> MKEFYISIETVGNNIVERYIDENGKERTREVEYLPTMFRHCKEESKYKDIYGKNCAPQKFPSMKDARDWMKRMERIGLEALGMNDFKLAYISDTYGSEIVYDRKFVRVANCDIEVTGDKFPDPMKAEYEIDAITHYDSIDDRFYVFDLLNSMYGSVSKWDAKLAAKLDCEGGDEVPQEILDRVIYMPFDNERDMLMEYINLWEQKRPAIFTGWNIEGFAVPYIMNRVKMILGERSMKRFSPIGRVKSKLIQNMYGSKEIYSIDGVSILDYLDLYKKFAFTNLPSFSLESVAQHETKKGKLPYDGPINKLRETNHQRYISYNIIDVESVQAIDKIRGFIDLVLSMS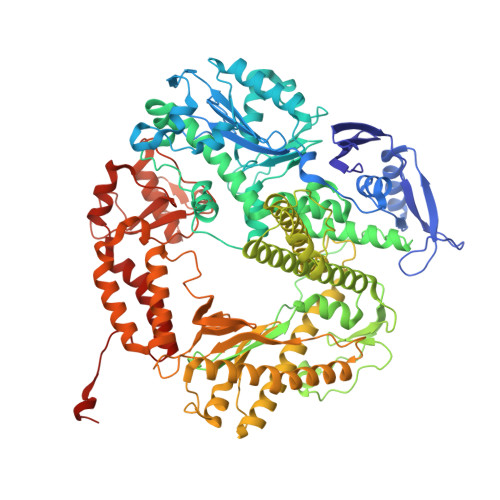YYAKMPFSGVMSPIKTWDAIIFNSLKGEHKVIPQQGSHVKQSFPGAFVFEPKPIARRYIMSFDLTSLYPSIIRQVNISPETIRGEFEVHPIHEYIAGTAPKPSDEYSCSPNGWMYDKHQEGIIPKEIAKVFFQRKDWKKKMFAEEMNAEAIKKIIMKGAGSCSTKPEVERYVKFSDDFLNELSNYTESVLNSLIEECEKAATLANTNQLNRKILINSLYGALGNIHFRYYDLRNATAITIFGQVGIQWIARKINEYLNKVCGTNDEDFIAAGDTDSVYVCVDKVIEKVGLDRFKEQNDLVEFMNQFGKKKMEPMIDVAYRELCDYMNNREHLMHMDREAISCPPLGSKGVGGFWKAKKRYALNVYDMEDKRFAEPHLKIMGMETQQSSTPKAVQEALEESIRRILQEGEESVQEYYKNFEKEYRQLDYKVIAEVKTANDIAKYDDKGWPGFKCPFHIRGVLTYRRAVSGLGVAPILDGNKVMVLPLREGNPFGDKCIAWPSGTELPKEIRSDVLSWIDHSTLFQKSFVKPLAGMCESAGMDYEEKASLDFLFG>[2x]MPQDPSTRSSPARLLIPEPRAGRARHAACVLLAVCFVVLFLSGEPLAPIIRSVCTQLAALQLGVLLKGCCCLAEE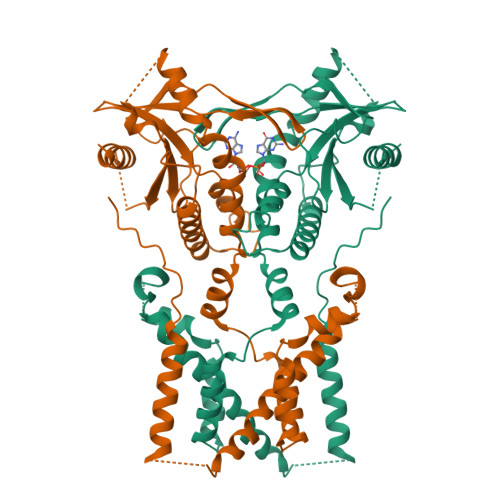IFHLHSRHHGSLWQVLCSCFPPRWYLALLLVGGSAYLDPPEDNGHSPRLALTLSCLCQLLVLALGLQKLSAVEVSELTESSKKNVAHGLAWSYYIGYLKVVLPRLKECMEELSRTNPMLRAHRDTWKLHILVPLGCDIWDDLEKADSNIQYLADLPETILTRAGIKRRVYKHSLYVIRDKDNKLRPCVLEFASPLQTLCAMSQDDCAAFSREQRLEQARLFYRSLRDILGSSKECAGLYRLIAYEEPAEPESHFLSGLILWHLQQQQREEYMVQEELPLGTSSVELSLQVSSSDLPQPLRSDCPGIHRPDYKDDDDK>MEGISIYTSDNYTEEMGSGDYDSMKEPCFREENANFNKIFLPTIYSIIFLTGIVGNGLVILVMGYQKKLRSMTDKYRLHLSVADLLFVITLPFWAVDAVANWYFGNFLCKAVHVIYTVNLYSSVLILAFISLDRYLAIVHATNSQRPRKLLAEKVVYVGVWIPALLLTIPDFIFANVSEADDRYICDRFYPNDLWVVVFQFQHIMVGLILPGIVILSCYCIIISKLSHSKGHQKRKALKTTVILILAFFACWLPYYIGISIDSFILLEIIKQGCEFENTVHKWISITEALAFFHCCLNPILYAFLGAKFKTSAQHALTSVSRGSSLKILSKGKRGGHSSVSTESESSSFHSSDYKDDDDK[4x];> KQFVTVFYGIPAWRNASIPLFCATKNRDTWGTIQCLPDNDDYQEIALNVTEAFDAWNNTVTEQAVEDVWNLFETSIKPCVKLTPLCVAMNCTRNMTTSTGTTDTQNITIINDTSPCVRADNCTGLKEEEMVDCQFNMTGLERDKRKQYTEAWYSKDVICDNNTSSRSKCYMNHCNTSVITESCDKHYWDAMRFRYCAPPGFALLRCNDTNYSGFAPNCSKVVAATCTRMMETQSSTWFGFNGTRAENRTYIYWHGKNNRTIISLNNFYNLTMHCKRPGNKTVLPIMSGFKFHSKPVINKKPRQAWCWFKGEWKEAMQEVKETLAKHPRYKGNRSRTENIKFKAPG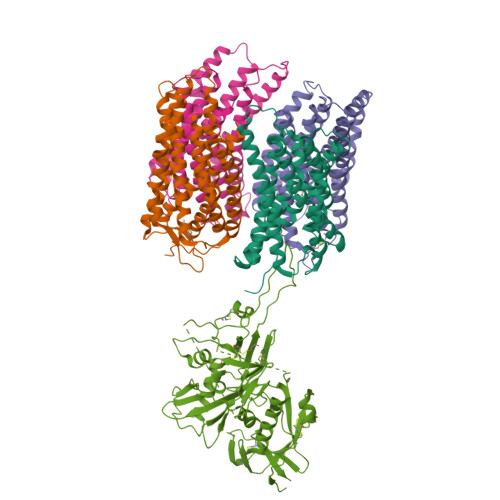RGSDPEAAYMWTNCRGEFLYCNMTWFLNWVDNRTGQKQRNYAPCHIRQIINTWHRVGKNVYLPPREGELTCNSTVTSIIANIDTGDQTDITFSAEVAELYRLELGDYKLVEITPIGFAPTSVKRYSSAHQRHTR>[2x]MEMTEYRQCVAKPISSSNPVGERLVDH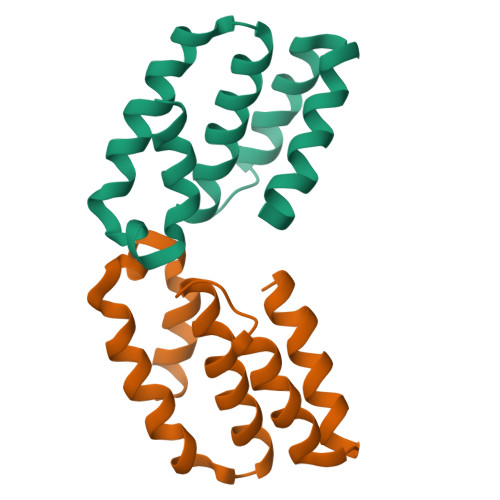PLFDFIEDQMMKVGSLSHASVQWDEVEHSTLKLLGEQSKDIKLLVYLLQCLHNQVTPTRLITSFAVMSEFLNQYWNDSYPAPGARGNLPRRKFFSQMAQRFTTVIEKFDFHHLDEADRQALQAAVEEWQQAVEKQGLSSELVESVVVRITAEIKRAEQRQQVTAQSSAERETPSAATSSPAASMVVDHSSDKAAKQTLLKVADFLAEQEFGIALSIRLRRFAVWGSITSLPDHKPDGETLLRGMQADRVKDYQDQLRHPDLALWRKVEQSLTMAPYWFEGQWMSYTIAQQLGKSDWCQAIAEETQQFLRRLPSLLELKFKGGEPFVSDSVKEWLASVGQSQGAAGQSVGGDWQEKRKEAFQLAKEGGIAVALSMLNDGLVSAVEPRDKFYWRLLSADLLRANHLDAMAGEQYQTLLNQVTTLSVPEWEPSLVEQIQRYTTSE>EELPAPVKAIEKQGITIIKTFDAPGGMKGYLGKYQDMGVTIYLTPDGKHAISGYMYNEKGENLSNTLIEKEIYAPAGREMWQRMEQSHWLLDGKKDAPVIVYVFADPFCPYCKQFWQQARPWVDSGKVQLRTLLVGVI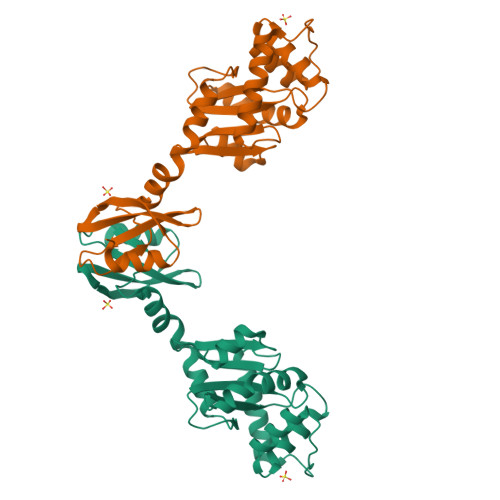KPESPATAAAILASKDPAKTWQQYEASGGKLKLNVPANVSTEQMKVLSDNEKLMDDLGANVMPAIYYMSKENTLQQAVGLPDQKTLNIIMGNKHHHHHH[2x]> MENTENSVDSKSIKNLEPKIIHGSESMDSGISLDNSYKMDYPEMGLCIIINNKNFHKSTGMTSRSGTDVDAANLRETFRNLKYEVRNKNDLTREEIVELMRDVSKEDHSKRSSFVCVLLSHGEEGIIFGTNG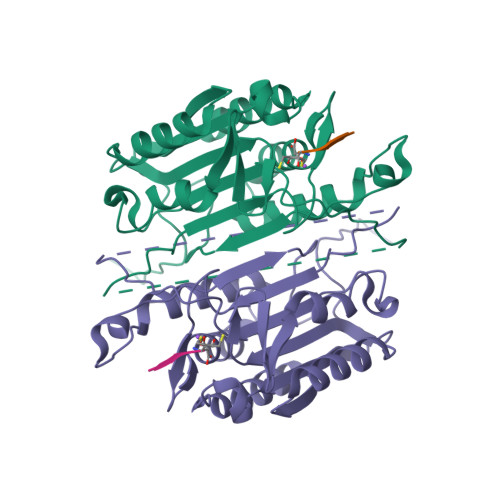PVDLKKITNFFRGDRCRSLTGKPKLFIIQACRGTELDCGIETDSGVDDDMACHKIPVEADFLYAYSTAPGYYSWRNSKDGSWFIQSLCAMLKQYADKLEFMHILTRVNRKVATEFESFSFDATFHAKKQIPCIWSMLTKELYFYHL> SNAEEERIERWVEQLREALIGDGFLLHYQPVLNLQGEPLELYQAFLRLERNGEMMSPNAFMAI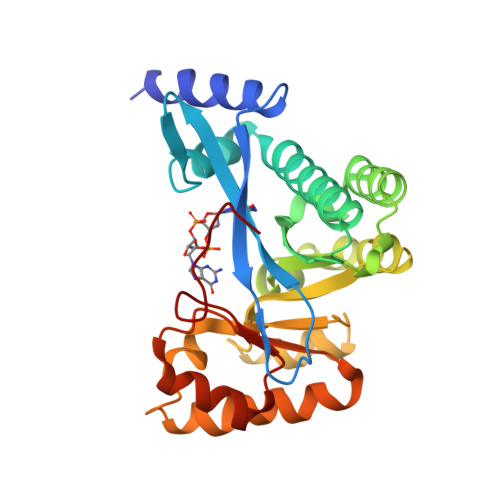AEEHDLITEIDRWVVARAIRQLGERQRAGHKTHLLVRIGPNSFSDPQMIDTIREQLAVYGVPGERLWLQTPESKVFTHLRNAQQFLASVSAMGCKVGLEQFGSGLDSFQLLAHFQPAFLKLDRSITGDIASARESQEKIREITSRAQPTGILTVAEFVADAQSMSSFFTAGVDYVQGDFVAPTGPLM>[4x]SNARVFNFAAGPATLPENVLLKAQADLYNWRGSGMSVMEMSHRGKEFLSIIQKAESDLRQLLEIPQEYSVLFLQGGATTQFAALPLNLCKSDDTVDFVVTGSWGDKAVKEAKKYCKTNVIWSGKSEKYTKVPSFEELEQTPDAKYLHICANETIHGVEFKDYPVPKNGFLVADMSSNFCSKPVDVSKFGVIYGGAQKNVGPSGVTIVIIRKDLIGNAQDITPVMLDYKIHDENSSLYNTPPCFGIYMCGLVFEDLLEQGGLKEVEKKNQRKADLLYNAIEESNGFFRCPVEKSVRSLMNVPFTLEKSELEAEFIKEAAKEKMVQLKGHRSVGGMRASIYNAMPLAGVEKLVAFMKDFQAKHA

PSATs are PLP-dependent enzymes that catalyze the second step of the phosphorylated pathway – reversible conversion of 3-PHP to PSer in a Glu-linked reaction. In this work, we describe a structure of the isoform 1 of chloroplastic PSAT from A. thaliana (At), which is further referred to in the manuscript as AtPSAT1. AtPSAT1 is a dimeric PLP-dependent AT that, similarly to other α-type ATs, binds the prosthetic group in the cavity within the large domain. The three crystal structures of AtPSAT1 present snapshots along the catalytic event showing PLP internal aldimine state, complex with PMP after the first half-reaction and PSer-PLP geminal diamine intermediate state.

Finally, crystallization of AtPSAT1 with 50 mM PSer and without sulfate ions in the crystallization conditions succeeded and the structure has shown somewhat unexpected results. The electron density maps revealed not only the position of PSer in the active site itself, but they also indicated the presence of two covalent bonds: between the nitrogen atom of PSer and C4′ of PLP, and between C4′ of PLP and Nζ atom of K265. The reaction snapshot in the AtPSAT1-PSer structure actually shows one of the reaction intermediates – the PLP-PSer geminal diamine. As a result of creation of two covalent bonds, the C4′ atom of PLP presents sp3 hybridization. In the PLP-PSer geminal diamine state, K265 and its neighborhood present almost identical conformation as in the internal aldimine state (the AtPSAT1-PLP structure). The bound PSer creates several hydrogen bonds in the active site, which include: a salt bridge between PSer carboxylate and guanidine group of R403 placed in the β14 strand, an H-bond between one of the oxygen atoms from the carboxyl group of PSer and N𝜀 of the indole ring of W171 from the α5 helix. Oxygen atoms from the phosphate group of PSer create several hydrogen bonds, either directly with protein side chains or through water molecules. These include direct hydrogen bonds with H396, R397 (loop between β13 and β14), and with R111∗, H110∗ (loop between η2 and α3). The superposition of AtPSAT1-PLP and AtPSAT1-PSer shows a pronounced movement of the loop 391–401 toward the catalytic site associated with PSer binding. Moreover, the structure of AtPSAT1-PSer shows the closed conformation of the gate-keeping loop between β13 and β14 (residues 391–401), required for the stabilization of AtPSAT1-PSer geminal diamine and most likely for the catalysis as well.> GETGQVIKSAVRSTVENTVQSTHSITTEATPALQAAETGATSNASDESMIETRNVVNTHGVAETSLEAFYGRAGLVAMFSTDGGIYRWYINFGEYVQLRAKLELLTYARFDMEFTIVAQVVNAQSKVQDFNVDYQVMFVPPGASVPENQDSYQWQSSCNPSVISNTGLPPARVSVPFMSSANAYSFSYDGYTQFGDASGSSYGIVPSNYLGMLVVRTCEDLDGTRLRVRVYAKPKHVKGWIPRSPRMTPYKSRYTGVYTDTTKFCANRARITTAG;> SAEACGYSDRVAQLTLGNSTITTQEAANIVVGYGRWPTSLRDTDATAVDKPTQPGVSAERFYTLPSVQWTNSFKGHYWKLPDALSELGLFGQNLQFHYLYRGGWVIHVQCNATKFHQGTLLVVATPEHKIQSAESPAFARTNPGEQGAAYQFPFTFEDGTALGNALIYPHQWVNLRTNNSATLVLPYVNALPMDSGIRHNNWTLSVIPIVPLEYAAGATTYVPITVTIAPMCTEYNGLRAAVTQ;> GIPTLYTPGSGQFLTTDDFQTPCMLPKFQPTPVIDIPGEVKNFLEVVQVESLVEINNVESAEGVARYRIPLNVQDAMDGQIMALRVDPGIDGPMQSTLLGVFTRYYAQWSGSLDFTFMFCGTFMTTGKVIIAYTPPGGDQPTNRRQAM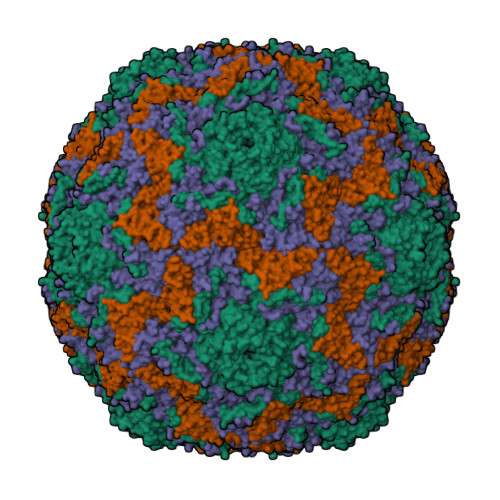LGTHVVWDFGLQSSITLVVPWISSGHFRGTTLENTIYKYRYYEAGYITMWYQTNMVVPPNFPTTASILMFVAAQPNFSLRILKDRPDISQEGALQ;> MGAQMSKNTAGSHTTGTYATGGSNIHYTNINYYENAASNSLNKQDFTQDPEKFTRPVVDVMKEAAVPLKSP> MSRKDYVLFDINTKAFVYGYQTNAIQRMLDFDYVCKRSSPSISAIINPSRAGIHKAFWGTKEIILPMYKTIPLAALAYPEADVMVNFASHRSAFETTMEALKEDTIRIVAVIAEGVPERQSRVMAATARKLDKIVIGPATVGGMTAGAFRIGNTAGTIENIIASKLYRPGCVGFVSKSGGMLNEAFNIISRNSDGIYEGVAIGGDRYPGSNMLDHILRYERNPAIKMIACLGELGGEDEYMIIQALKEKKITKPLVAWVT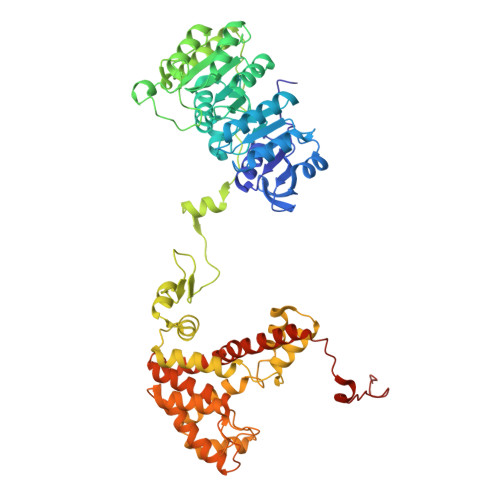GTCSPYLPASVQFGHAGAKANTEKETAQAKNDAFRQAGAYVPRSFDDYGEMVRQVYDMLLTRGIVQKFDEPEVPRIPTDYSKALATGDIRKPTTFICTISDDSGEELLYAGKKLSDVLDRKMGIGGVIGLLWFKKELPEYAAHFIELVIQIVADHGPAVSGAHNAIVASCAGKDLISSLCSGLLTIGPRFGGAIDDAAREFKRAQETGLAPEQFVGEMKKKGINIPGIGHKIKSVKNPDKRVQLLISYARANFPSTELLNYALQVEELTTAKKGNLILNVDGCIGILFIDLMSSCGAFSKEEIDEVVRLGYLNGLFALGRSIGLIGHILDQKRLGSRLYRHPAEDIAYMMPSEEEIQCKRDRGGSHHHHHH We present here an engineered chimeric PTP (ShufPTP) generated by shuffling the amino acid sequence of five extant hyperthermophilic archaeal PTPs. Despite ShufPTP’s high sequence similarity to its natural counterparts, ShufPTP presents a suite of unique properties, including high flexibility of the phosphate binding P-loop, facile oxidation of the active site cysteine, mechanistic promiscuity, and most notably, hyperthermostability, with a denaturation temperature likely >130 °C (>8°C higher than the highest recorded growth temperature of any archaeal strain). In each case, ShufPTP adopts a canonical architecture characteristic of the protein tyrosine phosphatase family, with particularly close structural similarity to its archaeal relatives TkPTP (RMSD 1.1 Å) and SsoPTP (RMSD 2.4 Å). The enzyme contains all four signature catalytic motifs that define modern PTPs: the phosphate-binding P-loop with conserved (H/V)CX5R(S/T) motif, the Q-loop that carries the water-directing glutamine, the IPD-loop that carries the conserved general acid (an aspartic acid), and the E-loop that carries a possible alternate general acid candidate (a glutamic acid).

The most striking difference between the ShufPTP structures is in the P-loop. We observe three distinct P-loop backbone conformations, which we designate “low,” “intermediate,” or “high,” referring to the relative position of the loop to the substrate binding site within the active site. Remarkably, the oxidation states of the catalytic nucleophile, C93 differ depending on the structure, often with multiple oxidation states observed in a single structure. Specifically, we observe the cysteine as: (1) a sulfenic acid, (2) a sulfonic acid, and (3) a rare cyclic five-membered sulfenamide ring (Figures 4B through F). The relationship between the P-loop conformation and the oxidation state of C93 is unclear, in part because multiple oxidation states are often observed in a single structure. In contrast, the phosphate binding loop of ShufPTP is highly mobile, taking on at least three distinct stable conformations, a feature that is highly uncommon in P-loop containing enzymes more broadly, given that phosphate binding P-loops tend to be structurally rigid and follow narrowly defined geometric parameters. Mechanistically, the active site cysteine of ShufPTP is readily amenable to oxidation, a feature that has emerged to be an important regulatory mechanism that links cellular tyrosine phosphorylation with signaling by reactive oxygen or nitrogen species. ShufPTP exhibits a higher oxidation rate than any of the previously reported values for PTPs, with a kinact of 65 ± 5 M−1 s−1.

> MWPSARFVDDNVAFSRMPTERELDEVAKDFDAVVVLVEEYELPYSLEEWKKRGVEVLHSPIPDFTAPSLEQLLEILRWIEARVREGKKVLIHCMGGLGRSGTVAVAWLMYSKGLPLREALRRVRSLRPGAVETYEQMEVLKELEKFLRSR> DERDRVQKKTFTKWVNKHLMKVRKHINDLYEDLRDGHNLISLLE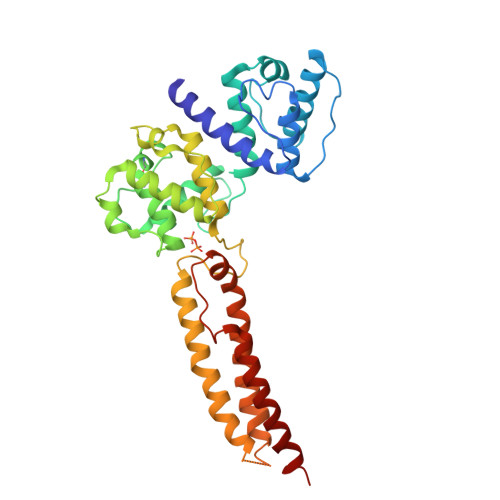VLSGIKLPREKGRMRFHRLQNVQIALDFLKQRQVKLVNIRNDDITDGNPKLTLGLIWTIILHFQISDIYISGESGDMSAKEKLLLWTQKVTAGYTGIKCTNFSSCWSDGKMFNALIHRYRPDLVDMERVQIQSNRENLEQAFEVAERLGVTRLLDAEDVDVPSPDEKSVITYVSSIYDAFPKVPEGGEGISATEVDSRWQEYQSRVDSLIPWIKQHTILMSDKTFPQNPVELKALYNQYIHFKETEILAKEREKGRIEELYKLLEVWIEFGRIKLPQGYHPNDVEEEWGKLIIEMLEREKSLRP> GSPKNYIEMKPHPWFFGKIPRAKAEEMLSKQRHDGAFLIRESESAPGDFSLSVKFGNDVQHFKVLRDGAGKYFL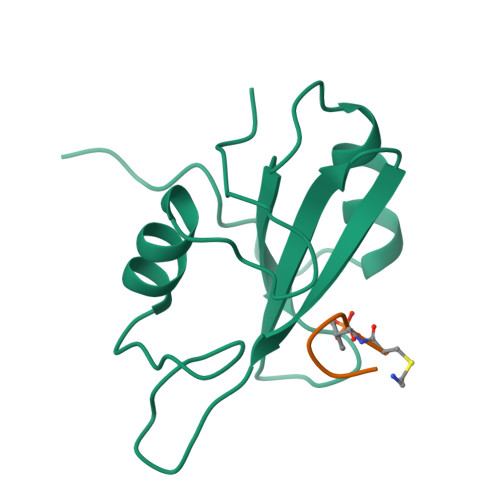WVVKFNSLNELVDYHRSTSVSRNQQIFLRDIEQVPQQPTYVQA;> XKYVNVP>MTERIRNVALRSKVCPAETASELIKHGDVVGTSGFTGAGYPKEVPKALAQRMEAAHDRGEKYQISLITGASTGPQLDGELAKANGVYFRSPFNTDATMRNRINAGETEYFDNHLGQVAGRAVQGNYGKFNIALVEATAITEDGGIVPTSSVGNSQTFLNLAEKVIIEVNEWQNPMLEGIHDIWDGNVSGVPTRDIVPIVRADQRVGGPVLRVNPDKIAAIVRTNDRDRNAPFAAPDETAKAIAGYLLDFFGHEVKQNRLPPSLLPLQSGVGNVANAVLEGLKEGPFE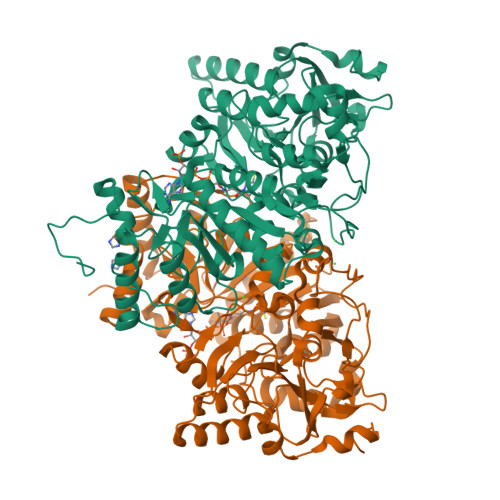NLVGYSEVIQDGMLAMLDSGRMRIASASSFSLSPEAAEEINNRMDFFRSKIILRQQDVSASPGIIRRLGCIAMNGMIEADIYGNVNSTRVMGSKMMNGIGGSGDFARSSYLSIFLSPSTAKGGKISAIVPMAAHVDHIMQDAQIFVTEQGLADLRGLSPVQRAREIISKCAHPDYRPMLQDYFDRALKNSFGKHTPHLLTEALSWHQRFIDTGTMLPSSLEHHHHHH[2x]>NAWDRTLIENGEKITSLH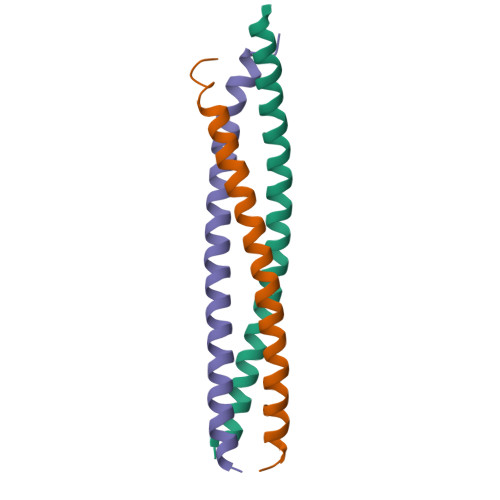REVEKVKLDQKRLDQELDFILSQQKELEDLLSPLEESVKEQSGTIY[2x];> GSHMTKQHQTRLDIISEDISELQKNQTTTMAKIAQYKRKLMDLSHRTLQVLIKQEIQRKSGYAIQ In order to elucidate their role in the lytic cassette of B. subtilis prophages, we cloned and produced XepA from the PBSX prophage and YomS from the SPβ prophage. The putative lysins XepA and YomS align very well, with a sequence identity of 38% (54% similarity) covering 85% of the overall sequence. The C-terminal disc of XepA is very similar to the structure of YomS, and the full-length protein including both domains is essential for cytotoxic activity. Both the XepA and YomS monomeric β-sandwiches adopt a fold resembling the C2 domain, which usually contains about 110 amino acids and 2–3 Ca2+ ions. In summary, we show that XepA initiates cell death in vivo, whereas YomS has no effect.

XepA crystallized from several conditions in multiple crystal forms. The crystal structures of the two highest diffracting crystal forms are reported here. XepA forms a remarkable pentameric structure in which two disc-shaped domains are connected by a linker region. Comparing the XepA structures in different crystal forms, only minor differences in the overall fold can be observed. A superposition of the whole pentamer of XepA crystal forms I and II resulted in an r.m.s.d. of 0.9 Å. However, using only the C-terminal pentamer disc of the different crystal forms to calculate the superposition matrix (r.m.s.d. of 0.3 Å), the molecule shows a domain motion in the tunnel and N-terminal disc corresponding to a rotation of 2.1°. Although it may be conceivable that high flexibility in the XepA linker region may permit a conformational change, for example a rotational movement of the C-terminal and N-terminal discs to open the pore area, this would require a major structural realignment. Comparisons with viral portal proteins show that the XepA tunnel has a relatively small diameter of approximately 10 Å, which suggests that it is too small to allow the entry of any DNA molecule (dsDNA, 20 Å; ssDNA, 15 Å).

>[5x]MVKYQYEFPLDKAGKAGAVKPYRGGKNDFVTPVSNLSGVAEILTNAALKATEAYSQLGQDRLGAVLISKVKGWAYADREGTLFIEESDNNNVWTTTAAVNVAAGVLTATDWVYLSKRYYRFRYVNGNLQQSEFVLYQSVGAGEMDVRVNEKTPLQIDFAENQTHDGRLKVEARKTFDFVFHENAESASEGAALPVDGAAHLLVEVYGTAEMSEVKFWGKSVSGQKLPIRGVKTDDATTASSTLGKAEAWAFDIKGFKEIIMEIISITGGTLSVKGTAVS>[4x]MHLRHLFSSRLRGSLLLGSLLVVSSFSTQAAEEMLRKAVGKGAYEMA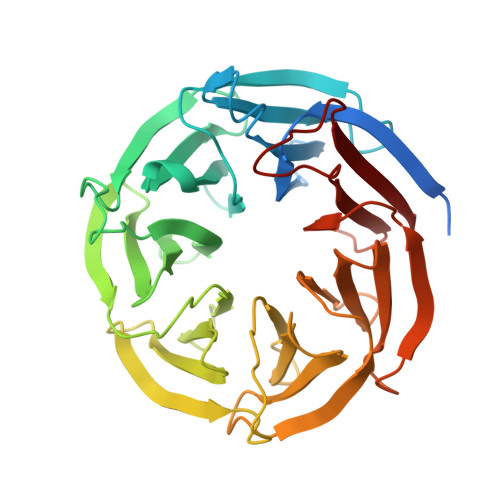YSQQENALWLATSQSRKLDKGGVVYRLDPVTLEVTQAIHNDLKPFGATINNTTQTLWFGNTVNSAVTAIDAKTGEVKGRLVLDDRKRTEEVRPLQPRELVADDATNTVYISGIGKESVIWVVDGGNIKLKTAIQNTGKMSTGLALDSEGKRLYTTNADGELITIDTADNKILSRKKLLDDGKEHFFINISLDTARQRAFITDSKAAEVLVVDTRNGNILAKVAAPESLAVLFNPARNEAYVTHRQAGKVSVIDAKSYKVVKTFDTPTHPNSLALSADGKTLYVSVKQKSTKQQEATQPDDVIRIAL>[2x]GMATSTDRTQEIQKLHELIKNIDYGMFTTVDDDGSLHSYPMSKSGDINSEATLWFFTYAGSHKVT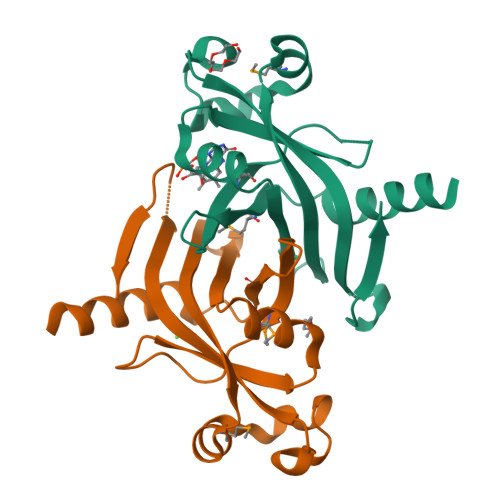EIEHHEQVNVSFSSPEQQRYVSISGTSQLVKDRNKMRELWKPELQTWFPKGLDEPDIALLKVNINQVNYWDSTSSFKPQTISF4-chloro-N'-[(1E)-(3,5-dibromo-2,4-dihydroxyphenyl)methylidene]benzohydrazide | C14 H9 Br2 Cl N2 O3 | 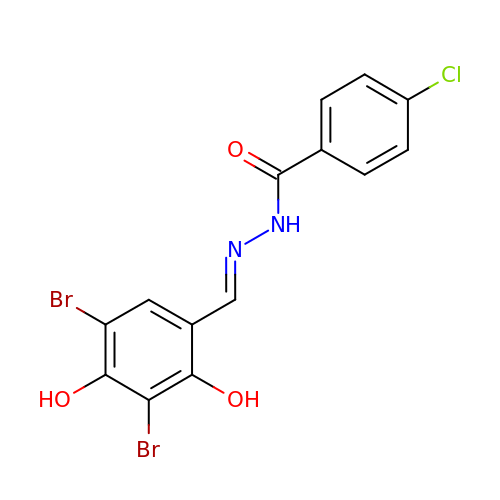ZDMUFSJTENTNDA-NGYBGAFCSA-N>AQVINTFDGVADYLQTYHKLPDNYITKSEAQALGWVASKGNLADVAPGKSIGGDIFSNREGKLPGKSGRTWREADINYTSGFRNSDRILYSSDWLIYKTTDAYQTFTKIR[3x];>[3x]MKKA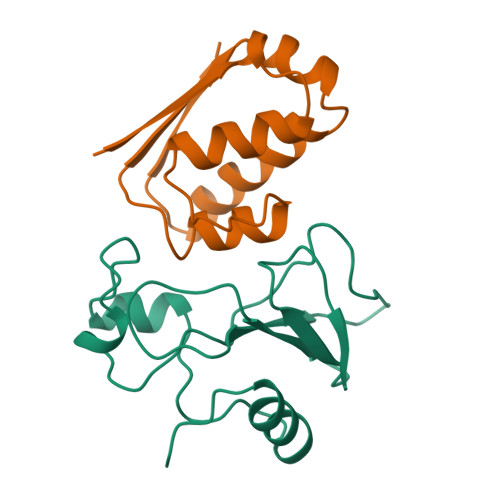VINGEQIRSISDLHQTLKKELALPEFYGENLDALWDCLTGWVEYPLVLEWRQFEQSKQLTENGAESVLQVFREAKAEGCDITIILS>[4x]METLLVVGAGPKALAVAAKSHVLRQLGLSAP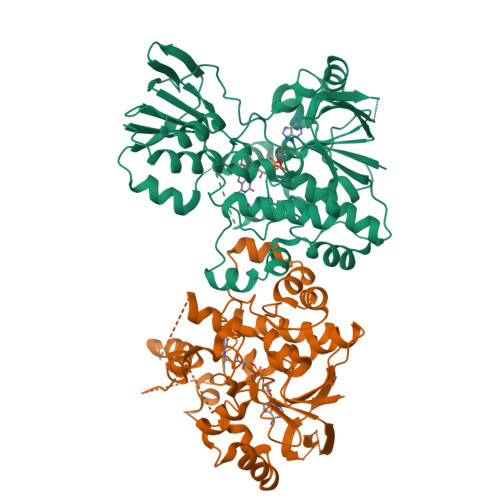RVIAVEAHAVGGNWLASGGWTDGRHRLGTSPEKDIGFPYHSTWARGHNREINEAMMAFSWTSFLVEHGTYAEWIDRGRPSPQHHVWAKYLQWVARKIDLELVLGKVRTIRQRPTDGGAGWSVEVAGADGATTELEADGLMITGPGQSTKALAAHPRVLSIAEFWDLAGKRKLPISSRAAVIGGGETAGSALDELVRHEMLTISVISPMATIYTRGESYFENSLFSDPTKWNALSIQERRDVIRRTDRGVFSVRVQESLLGDNRVHHLQGRVTRIVGQGDGVAVTLRNEMRADQVHNFDLVVDATGGQPLWFLDLFDSESADLLELAVGGPLTQQRIESSIGYDLAVTGLGAKLYLPNMAALAQGPGFPNLSCLGELSDRVLRAEPARVRAGARQLAAQ>MEPQREFFHIAGRSAKEYLSENLVQFIQATQNYFNIGEKFRDPYVAPSAGVTTDRSQKLQLRVVPIQTEDNVNYYKARFTLNVGDNRLVDLGSSYFDIKGTLDRGPSFKPYGGTAYNPLAPKSAPINSAFTVGNDTHFVAQLPQTYAAGGTGVTEAIQQQVSGVDPNPQVGQPNYAGPVVVNTTNNAGLGRIVSADSEGQQFPCYGAYAPPQSAGGDVSTAAVTKTYINTTNNNGRVSGTMATDTITWENPDAHFADFVDDRRATAAGNRPNYIGFRDNFIGMMYYNSGSNTGSFSSQTQQLNIVLDLNDRNSELSYQYLLADLTSRWHYFALWNQAVDDYDHHVRILENDGYEEGPPNLAFPPHVISNPFAPAAVGTGMTVNEQQQTAAVTANTVALIGYGNIPAVEMNLPANLKRTFLYSNVAMYLPDTYKFTPANVDLPENHLSYGYINGRLPLPNIVDTWTDIGARWSLDVMDTVNPFNHHRNTGLKYRSQLLGNGRYCDFHIQVPQKFFAIKNLLLLPGTYNYEWYFRKDPNMVLQSTLGNDLRADGASITYTQINLYVSFFPMNYDTQSELELMLRNATNDQNFSDYLGAVNNLYQIPAGSSTVVVNIPDRSWGAFRGWSFTRLKVSETPRIGATQDPNFQYSGSIPYLDGTFYLSHTFQRCSIQWDSSVPWPGNDRMLTPNWFEIKRPINQDAEGNDTMQSNLTKDFFMVQMAASYNQGYQGFNWPNCTKHYGFINNFEPMSRQVPEYGANYPNLMAAYLANPQTMPIWNNCGFQQKTATNVLLERCGHPYVANWPYPLSGRNAVPNQVTERKFLVDRYLWQIPFSSNFLNMGTLTDLGQNVMYANSSHSLNMQFTVDPMTEPTYLMLLFGVFDQVVINQPTRSGISVAYLRLPFASGSAAT[12x];> MEVYVPPPRVMAPTEGRNSISYNPIAPLQDTTHIYIIDNKTSDIENLNIHKDHSNFYTNIVQNVDVAPSDAATQTIKLDERSRWGGELHTILKTNAPNVTEFFNSNSFKALLMSDKTDPANPVYTWFELSIPEGDYTVGSLIDMLNNAVVENYLEVGRQKGVQISDIGVKFDTRNFSLGRDPLTSLVTPGNYTFKAFHPDIVLLPGCGVDFTHSRINNMLGMRKRFPYEPGYVITYEDLVGGNIPALLDLAKYPGETSPVLQDPDGNSYHVEEVSPKKWQTKYRSWCLAYNSSQGTLKSEQILTVPDITGGLGQLYWSLPDAFKPPVTFTNNTTDISTQPVTGMHLFPLSQRIVYNTSAVYAQLVEQMTNNTKVFNRFPKNAILMQPPYDTTQWISENVPYVADHGIQPLKNSLTGVQRVTLTDDRRRSCPYIYKTLATVTPKVLSSATLQ;> MDPGLKPSSLWTHKIIDSIIANRSLSAVQNFRKQPLANKLTALEDAIVQPRKDTTPETVAAILQELVAMGALQPNEVGPMFSDLMIRVHKYNSTNVQNNLSVLLGDIRAAQSEAIRSTNVGELSNQVVLNDFLSREPAVVPQGQHNYEAFKQTLRLMVNEAPNVTLFKSGPDTLMQVNIRGVNTVNLNSAFKNLKNFWGVQLDTEIVPGSISSKLSSNTRVLLLFLAPFTNDSTFTPDTFISQIMRLYRETVAASIEQPQETELEVAETIRELGGDVEDIGRTMAFLLKNKEEIVSNPRTLSPRQLNVLRYVQESLQDRIDRNGEEPEDALRNLVFSFAPSYFEANGPFIRRLISYLEVALINSPNYFREIYSNKYWTPPASFWTQNYGDFHLEREAEAERRAASEAGYGDFEEGDFALPDNLGEGSDLAWDDFNTAMSPSVPPTPSVRSAPASLSYGRTSPSSVSSLTASDRNIGATLARAVIPPAAAAIGSAAGEALYPSLGQYLAPAASLAATRLLNLTRARRQRLKRDSLARHRRITEVRGVYPKAAPTRSSSSSSVSSTPTVFEPLPGAFSVINPLMRPEGDRDVSGTGIVNPFSHLKPRNGLQ;>MDAPVTPYIWQYQPQTGKAAGARQNYGAVINWLSADNNMFHRVQTVNRARNLIDEIREETVRPDLAASFNDWTYDQLTQPPGTAYLPAPDPLTGPTTIRDKVLSAEGEQLAGSRPSVLHGGASLPPSAYSLGDGREYMKLTRDALPFPQNWMVKENGVWTPIVEQRAALRGGSANALSSYPTLLFNQPPILRYRRPGQQLQGSGVIAPSSKVLSLLSEAPR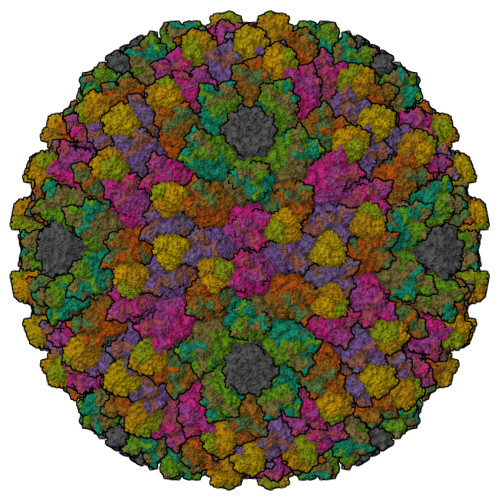IPRTEGMTPYQFANSFPPVVYEDPFSQNLAVFPKEFSPLFEPENQVLASSLATLQYN[2x];>MTSVEELYVINPINQWPAPGSFSSQKPPGTLLPGEDPEAVFKQYHVVYLVPGAQYHWKNILIEKPVWIYGNGATVRTSGTGPILRIVGNRTEKRDVRIQDISFFGEDCTPNRMEPMSEKLVYQMAIWVTDMKRVTIKGCNFTNFAGAAVFFEETAYNGFFWSMQHLITECRFTGCRIGIANGGRSEYSTASFNNFFDCQICFNVVGGNWNRCGNIAANCRCVYLHTTNMWYEGAGGNFNAAHGSFTGNTMNHCDYGGNLWPTAFQLPDREIQLAGFYFDNARARCPTWTGNTQYYGDMKILNFNQANDAAIFVIDGCALYGQPGDTGSIETTAALTDKVFIQGCQGNKVTLFNIKAANVVPAIGTIKQKP[4x]>MYTLNWQPPYDWSWMLGFLAARAVSSVET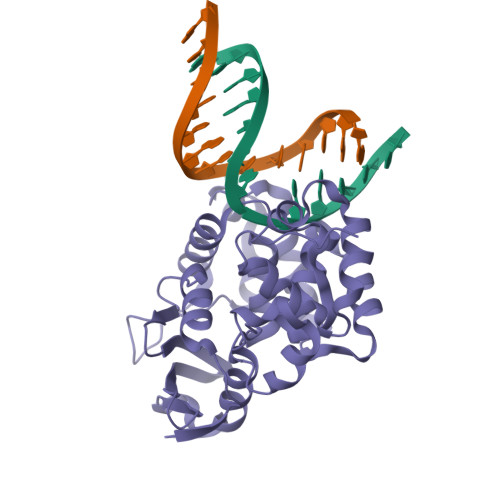VADSYYARSLAVGEYRGVVTAIPDIARHTLHINLSAGLEPVAAECLAKMSRLFDLQCNPQIVNGALGRLGAARPGLRLPGCVDAFEQGVRAILGQLVSVAMAAKLTARVAQLYGERLDDFPEYICFPTPQRLAAADPQALKALGMPLKRAEALIHLANAALEGTLPMTIPGDVEQAMKTLQTFPGIGRWTANYFALRGWQAKDVFLPDDYLIKQRFPGMTPAQIRRYAERWKPWRSYALLHIWYTEGWQPDEA[2x]oxo{[(1S)-1-phenylethyl]amino}acetic acid | C10 H11 N O3 | 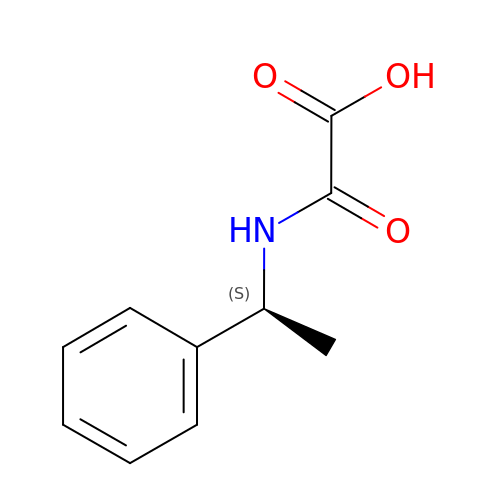RVIXKSXCAWSWSX-ZETCQYMHSA-N beta,beta-carotene-4,4'-dione | C40 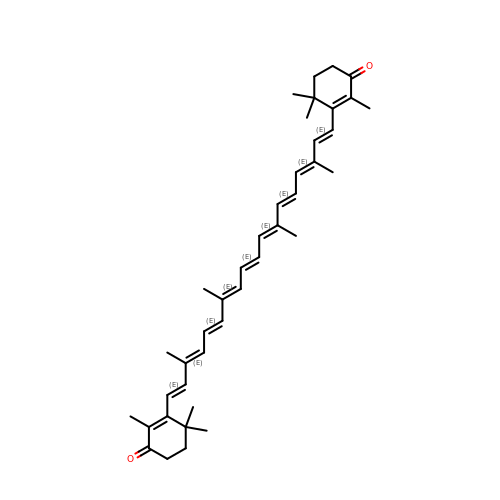H52 O2 | FDSDTBUPSURDBL-DKLMTRRASA-N> MVADNIDAGVAIAVADQSSSPVGDKVELPAGNYILVGVDIDTTGRRLMDEIVQLAAYTPTDHFEQYIMPYMNLNPAARQRHQVRVISI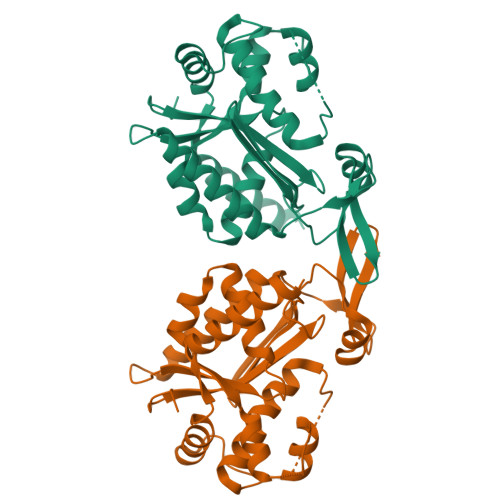GFYRMLKSMQTYKIIKSKSEIAALKDFLNWLEQLKTKAGPSSDGIVLIYHEERKFIPYMILESLKKYGLLERFTASVKSFANSINLAKASIGDANIKNYSLRKLSKILSTTKEEDAACSASTSGSGSGLGSGSSMVSDSVSISPRDSTVTNGDDKQSSKNAVQGKRELFDGNASVRAKLAFDVALQLSNSDGKPEPKSSEALENMFNAIRPFAKLVVSDVLELDIQIENLERQNSFRPVFLNYFK>[2x]MRSRRVDVMDVMNRLILAMDLMNRDDALRVTGEVREYIDTVKIGYPLVLSEGMDIIAEFRKRFGCRIIADFKVADIPETNEKICRATFKAGADAIIVHGFPGADSVRACLNVAEEMGREVF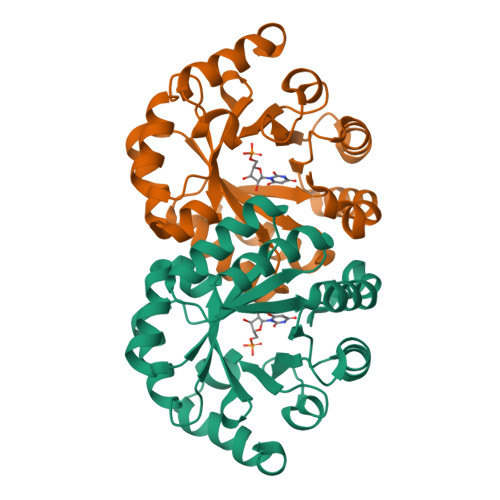LLTEMSHPGAEMFIQGAADEIARMGVDLGVKNYVGPSVRPERLSRLREIIGQDSFLISPGVGAQGGDPGETLRFADAIIVGASIYLADNPAAAAAGIIESIKDLLNP5-OXO-L-NORLEUCINE | C6 H11 N O3 | 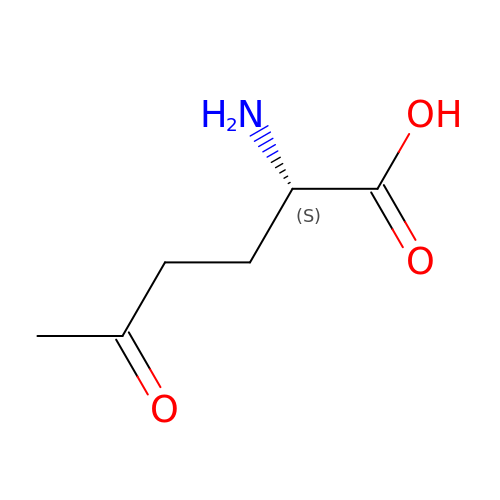KSIJECNNZVKMJG-YFKPBYRVSA-N> DVDKNDLKKKSDIDSSKLFNLTSYYTDITW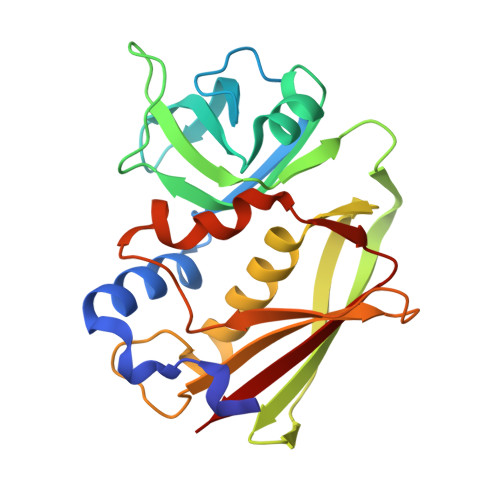QLDESNKISTDQLLNNTIILKDIDISVLKTSSLKVEFNSSDLANQFKGKNIDIYGLYYGNKCVGLTEEKTSCLYGGVTIYDGNQLDEERVIGVNVFKDGIQQEGFVIKTKKAKVTVQELDTKVRFKLENLYKIYNKDTGNIQKGCIFFHSNNHQNQSFYYDLYNIKGSVGAEFFQFYSDNRTVSSSNYHIDVFLYKD> MATDVAQGPNGRALAESMNPDLLSAIQQHISIERYASVTYLAMSIWCAERELAGFYQFFDGEAKDEQSHAVHFTQYLIARSQSNDLQTLDAPRQNWDSLASLMATAFQMEADTTSSIQSVYALAERNSDTRTTVFLDPLIDAQIQSEDQFAYLLGRVKFANGDPTALLVIDNELRAGQTQRG

Ferritins are proteins forming 24meric rhombic dodecahedral cages that play a key role in iron storage and detoxification in all cell types. Their function requires the transport of Fe2+ from the exterior of the protein to buried di-iron catalytic sites, known as ferroxidase centres, where Fe2+ is oxidized to form Fe3+-oxo precursors of the ferritin mineral core. SynFtn, isolated from the cyanobacterium Synechococcus CC9311, is an atypical prokaryotic ferritin that was recently shown to take up Fe2+ via its threefold channels. The wild-type protein contains three iron binding sites: high- and low-affinity binding sites at the FOC, sites 1 and 2, respectively, and site 3 located in the threefold channel and coordinated by the side chains of three symmetry equivalent Asp137 residues.

To probe the possibility that Glu141 of SynFtn acts as a ‘transfer’ carboxylate with equivalent function to the conserved carboxylates of the animal ferritins, two variants, E141A and E141D, were generated. Variants E141A and E141D both crystallized under conditions identical to those reported for wild-type SynFtn. Protein structures derived from all crystals harvested without iron enrichment were free of bound metal ions, as expected. The structures of variants E141A and E141D overlay with that reported for the wild-type protein with overall rmsd (for main chain atoms) of 0.10 and 0.11 Å, respectively, with the major difference in structure being associated with the side chain of the substituted residue. Typically when site 3 is vacant, residue 141 is oriented toward the FOC. This is the case for the metal-free structure of variant E141D, while conformational flexibility at this position is not possible in E141A. In contrast, the rate constant for iron binding to the E141D variant was almost identical to the wild-type protein, at 3.4×105  m −1 s−1, demonstrating that the conservative replacement of Glu by Asp did not have a significant effect on oxidation rate. Consistent with this, variant E141D was able to bind, oxidize and mineralize iron all at similar rates to the wild-type protein, despite the lack of any crystallographic evidence for conformational flexibility of Asp141. It appears, therefore, that the charge of the carboxylate group is of greater importance for SynFtn function than the observed conformational flexibility of residue Glu141, despite the altered fractional occupancy of SynFtn iron binding sites induced by the E141D substitution.N-(ETHYLSULFONYL)TRYPTOPHYL-N~1~-{4-[AMINO(IMINO)METHYL]BENZYL}GLUTAMAMIDE | C26 H33 N7 O5 S | 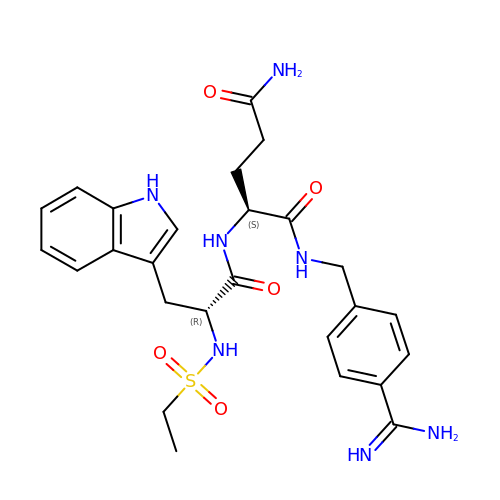FJGWLOKDOKYXMU-FCHUYYIVSA-N> MSLEALMNVQFFDHAHHKLKIRGLQSPVDVLTFEGREQLSTPFRYDIQFTSSDKAIAPESVLMQDGAFSLTAPPVQGMPVQTALRTLHGVITGFKHLSSSQDEARYEVRLEPRMALLTRSRQNAIYQNQTVPQIVEKILRERHQMRGQDFVFNLKSEYPAREQVMQYGEDDLTFVSRLLSEVGIWFRFATDARLKIEVIEFYDDQSGYERGLTLPLRHPSGLFDGETEAVWGLNTAYSVVEKSV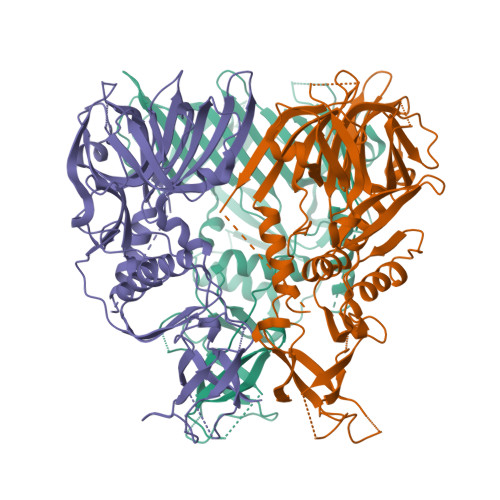STRDYNYREATAEMTTGQHDATGGDNTTYGEAYHYADNFLQQGDKEAAESGAFYARIRHERYLNEQAILKGQSTSSLLMPGLEIKVQGDDAPAVFRKGVLITGVTTSAARDRSYELTFTAIPYSERYGYRPALIPRPVMAGTLPARVTSTVKNDIYAHIDKDGRYRVNLDFDRDTWKPGYESLWVRQSRPYAGDTYGLHLPLLAGTEVSIAFEEGNPDRPYIAGVKHDSAHTDHVTIQNEGHHHHHH>[2x]MTVSRRGFMAGLALTGAAALPVAYYTHRHLTREEEPQTPDEASLDLAATDGIRLGDRLRGLWDLRLVGGDAELPGLPREGLQLVLDVAPKGRGLIGY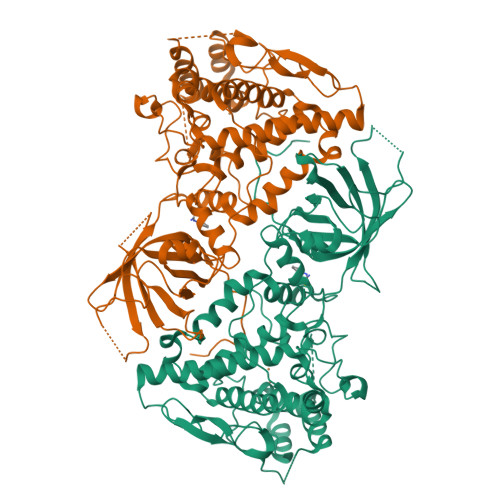LDTPERLLAAEPPRFRVLGDLLGASSASIRWRLVDQASGSVAPTHDCSAVFDEVWADYANAGDGTLSGRIQRLERSPLSPNEDFRFVAVKRHFPLAHERIVLNEKLLGWLVSPQHRLFHQLWHASRDKWHRLSEKQRNALRGVGWQPGPLDRERDARGPRKDRNASGIDFFFMHRHMLHTARSMQDLPSWERLPRPVVPLEYDRPGFIRYFDNPDGFSVPPAWVAVDDDEYSEWLHGLKSAEAYHANFLVWESQYQDPAYLAKLTLGQFGSELELGMHDWLHMRWASVTRDPSNGAPVMTDRFPADFAPRWFRPENDFLGDPFSSHVNPVFWSFHGWIDDRIEDWYRAHERFHPGEVQRREVEGIQWFAPGRWVEVGDPWLGPATHGCGLSDVQASSNSVELDVETMKLALRIIFSEEDQLSGWLKRAPRRPWYARNLKLARDQLRR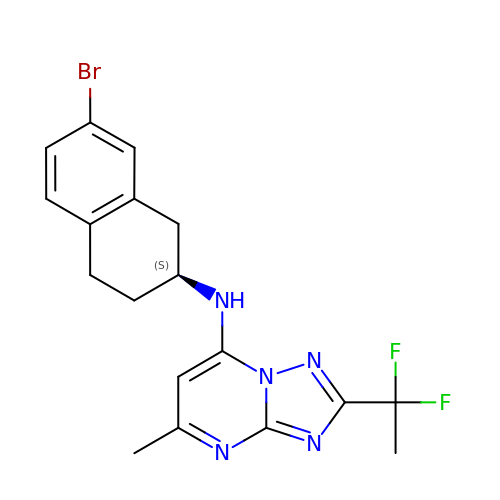2-[1,1-bis(fluoranyl)ethyl]-~{N}-[(2~{S})-7-bromanyl-1,2,3,4-tetrahydronaphthalen-2-yl]-5-methyl-[1,2,4]triazolo[1,5-a]pyrimidin-7-amine | C18 H18 Br F2 N5 | WSMWEZWUWJDREU-AWEZNQCLSA-N>MIKKAVLPVAGLGTRFLPASKSIPKEMVTVVDRPAIEYVVREAVEAGIEQIILVTHSSKASIENYFDRNFELETTLEQKKKFDLLAEITQIVPE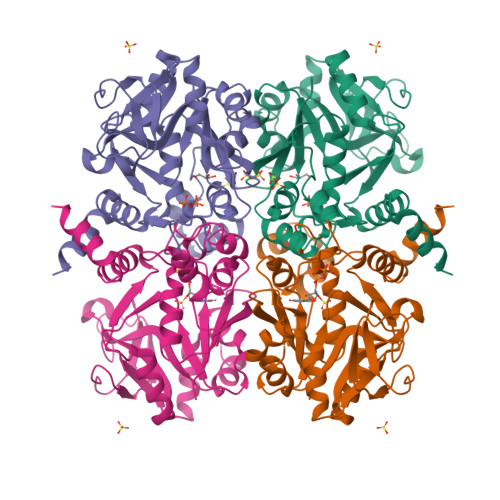HVSVISVRQPQPLGLGHAVLCAKSVVGEDDFAVLLPDVLVKDGSGQNDLSRMISRYNSSQAAQIMVEAVPDHLVDQYGIVDVAQSPNEGESIAMQGIVEKPPVGAAPSNLSVVGRYVLPAKIMQLLENTPKGAGNEIQLTDAIAMLQDTDTVEAYRMQGQTFDCGSKLGYLKAVLHYGLEHPKLGMEFKQLILELK[2x]>GPLGSDLKDAEAVQKFFLEEIQLGEELLAQGDYEKGVDHLTNAIAVCGQPQQLLQVLQQTLPPPVFQ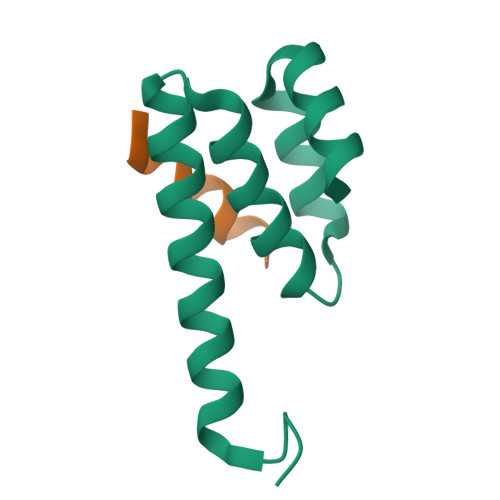MLLTKL[2x];>[2x]GPRLSRLLSSAGC> QYFMTE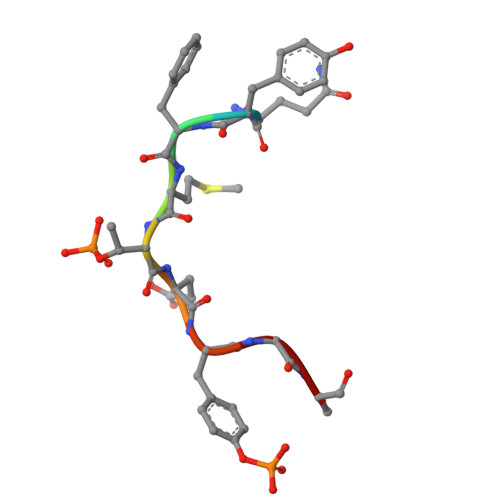YVA> GSHMLGERLGIPAPRRIEAFDNSNIYGADPVSALVVFLDGKPAKKEYRKYKVKTVAGPNDYETMREVVRRRYTRVLKEGLPLPDLIIIDGGKGHLSAVRDVLENELGLDVPLAGLAKDEKHRTSELLAGDP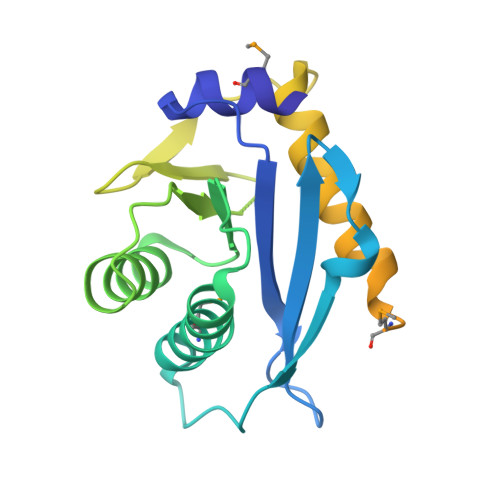PDVVPLDRQSQEFYLLQRIQDEVHRFAVMFHRKTRQKTMFHSVLDDIPGVGEKRKKALLNYFGSVKKMKEATVEELQRANIPRAVAEKIYEKLHE> GSHMNTAEEDMEDDTSWRSEATFQFTVERFSRLSESVLSPPCFVRNLPWKIMVMPRFYPD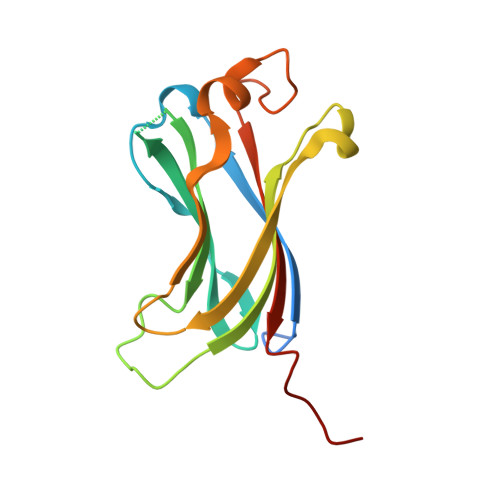RPHQKSVGFFLQCNAESDSTSWSCHAQAVLKIINYRDDEKSFSRRISHLFFHKENDWGFSNFMAWSEVTDPEKGFIDDDKVTFEVFVQADLDAGVSEHS RNF125 is a small protein (25 kD) that contains, in addition to the RING domain, three zinc fingers (ZnFs) and a ubiquitin interacting motif (UIM). RNF125 was first identified as a regulator of T cell activation, but has also been shown to negatively regulate the cytoplasmic viral RNA sensors RIG-I and MDA526, to interfere with HIV transcription27 and promote p53 degradation. Using mutational analysis, activity based assays, NMR and X-ray crystallography, we have demonstrated the essential role of a C2HC ZnF for the interaction of RNF125 with the E2, which originates from the requirement of the C2HC ZnF for the structural stability of the RING domain. Collectively, our experiments show that the RING and C2HC ZnF domains with their linker regions act as a functional unit held together by interdomain contacts.

However, the structure of the truncated RNF125stop129 was solved at a resolution of 1.55 Å. RNF125stop129 shows a compact module in which the RING domain and the C2HC ZnF are easily discerned. The predicted unstructured N-terminal 30 amino acids were not observed in the electron density. The C2HC ZnF adopts a ββα fold, typical for ZnF domains, which is capped on both sides by α-helices formed by regions Li1 and Li2120-128. The α-helix of Li2120-128 is almost continuous with that of the C2HC ZnF, but is kinked at C119. As expected, C100, C103, H115 and C119 coordinate the Zn atom. Interestingly, the structure demonstrates that extensive intramolecular interactions take place between the RING domain and the C2HC ZnF. Specifically, electrostatic interactions can be observed between C57 coordinating the proximal Zn2+ of the RING domain and R113 in the C2HC ZnF, where R113 makes additional hydrophobic contacts with H45 in the RING domain. Furthermore, a hydrophobic patch is formed between V43 in the RING, and L109/M112 in the C2HC ZnF. Additionally, an anchor between the RING and Li2120-128 is provided by a strong hydrogen bond (2.6 Å) between E42 Oε2 and the hydroxyl group of Tyr122.

>MGSVLSTDSGKSAPASATARALERRRDPELPVTSFDCAVCLEVLHQPVRTRCGHVFCRSCIATSLKNNKWTCPYCRAYLPSEGVPATDVAKRMKSEYKNCAECDTLVCLSEMRAHIRTCQKYIDKYGPLQELEETAARCVCPFCQRELYEDSLLDHCITHHRSERRPVFCPLCRLIPDENPSSFSGSLIRHLQVSHTLFYDDFIDFNIIEEALIRRVLDRSLLEYVNHSNTT[2x]>RHDYAPLRLYIDGRFHDADGRRTQPVVDPGTTRVLGELPHATAHDIDAAVQAAHRAFVTWRHESPLVRSDLLRRAAALARERAETIGRHITMDQGKPLREAIAEVVSAAEQLEWHAEEGRRTYGRVVPARSPDVMQTVLREPIGVCAAFSPWNFPFSQAMHKIAAALASGCTLVLKGPEESPSAIVALAQLFHDAGLPPGCLNIVWGVPGDVSKQLIEAPQVRKISFTGSVPVGKQLAALAASLMKRMTMELGGHAPVLVCADADVERAAAMLAAYKFRNAGQVCVSPTRFFVQRAAFDRFVCAYLD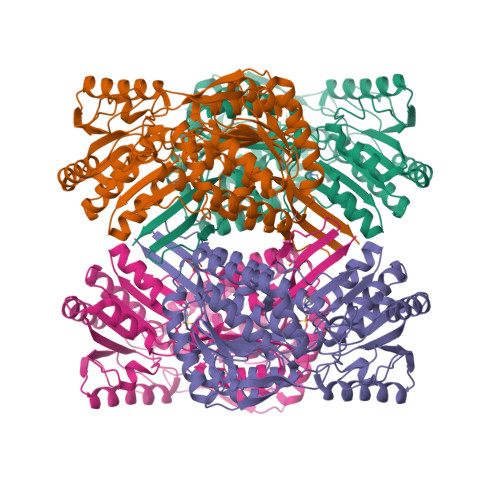AVGTIRVGYGLDAGVTMGPLAHARRVDEIDAFVADATAKGAQIATGGMRLPGPGHYFAPTVVLGPTRDTRLMNDEPFGPIVGIVPFDDLDDALAEANRLPFGLASYAFTTSARNAHRISRALEAGMVNINHFGMGPAEIPFGGVKDSGFGSEGGMEAFDGYLVTKFVTQMN[8x]> MSKTDWNASGLSRPSPSAHWPSRKLWQHGQKYQTTQDRSEPPAGKRRQAV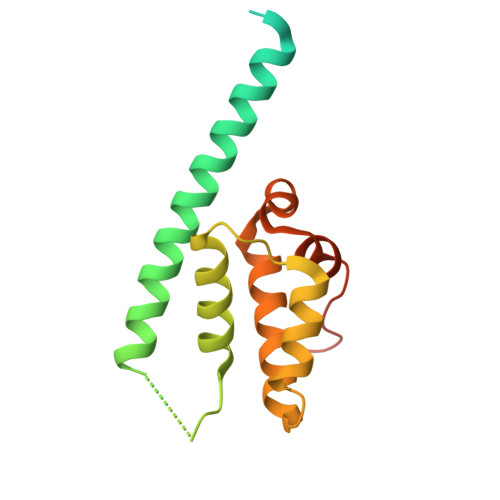RVSANHASQQLDQLKAVHLASAVRDLERAMTTLKLWESPQEISRHQALGYSVIMFMITAVKRLRESKMLTLSWFNQALMVIAPSQEETMNLKTAMWILANLIPRDMLSLTGDLLPSLWGSGLLMLKLQKEGRSTSS> MEEVVLITVPSEEVARTIAKALVEERLAACVNIVPGLTSIYRWQGEVVEDQELLLLV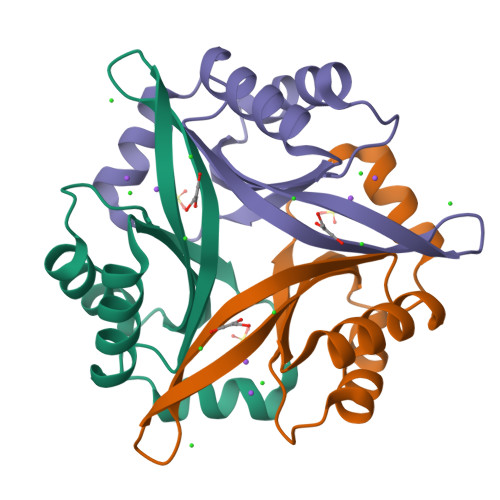KTTTHAFPKLKERVKALHPYTVPEIVALPIAEGNREYLDWLRENTG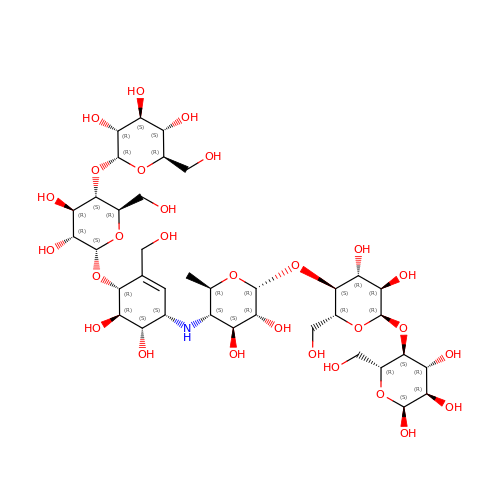ACARBOSE DERIVED HEXASACCHARIDE | C37 H63 N O28 | HAWINQMQXQMONI-OBPZNAFQSA-N> SVFAYESSVHSTNVLLSLNDQRKKDVLCDVTIFVEGQRFRAHRSVLAACSSYFHSRIVGQADGELNITLPEEVTVKGFEPLIQFAYTAKLILSKENV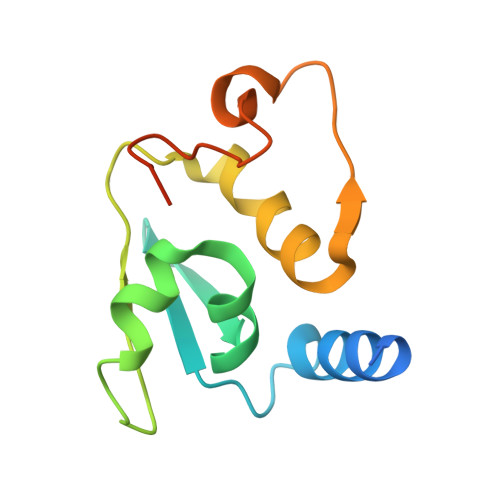DEVCKCVEFLSVHNIEESCFQFLKF>[5x]DYKDDDDK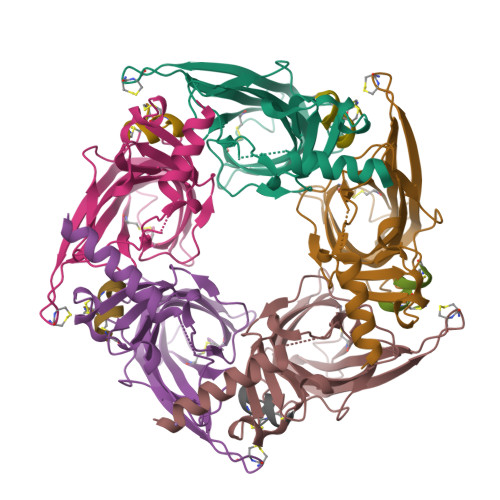LHSQANLMRLKSDLFNRSPMYPGPTKDDPLTVTLGFTLQDIVKADSSTNEVDLVYYEQQRWKLNSLMWDPNEYGNITDFRTSAADIWTPDITAYSSTRPVQVLSPQIAVVTHDGSVMFIPAQRLSFMCDPTGVDSEEGATCAVKFGSWVYSGFEIDLKTDTDQVDLSSYYASSKYEILSATQTRQVQHYSCCPEPYIDVNLVVKFRERRAGNGFFRNLFDSR;>GCCSTPPCAVLYCX[5x]> MKSASDPFDLKRFVYAQAPVYRSVVEELRAGRKRGHWM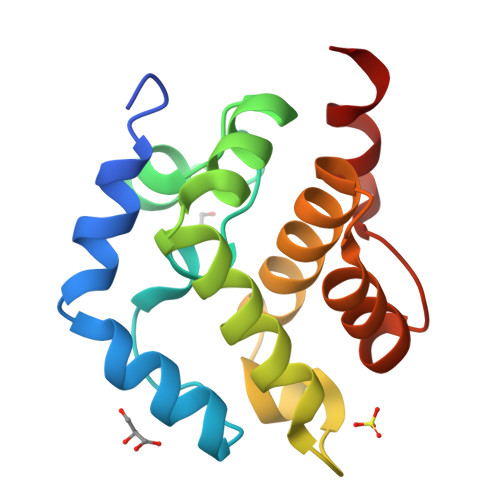WFVFPQLRGLGSSPLAVRYGISSLEEAQAYLQHDLLGPRLHECTGLVNQVQGRSIEEIFGPPDDLKLCSSMTLFARATDANQDFVALLAKYYGGGEDRRTVALLAVT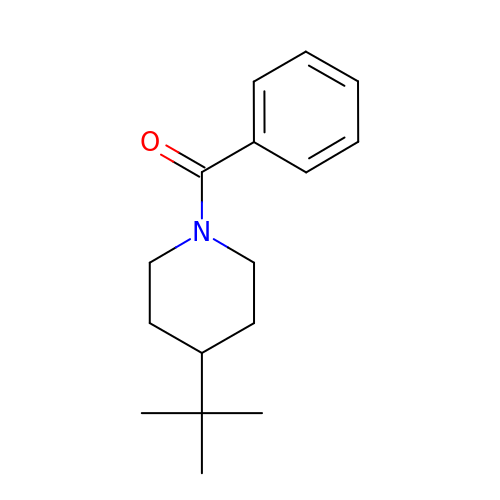(4-tert-butylpiperidin-1-yl)(phenyl)methanone | C16 H23 N O | UVPFTRNYXLMKBI-UHFFFAOYSA-N>STRPPRFQRDFVDLRTDCPSTHPPIRVMQWNILAQALGEGKDNFVQCPVEALKWEERKCLILEEILAYQPDILCLQEVDHYFDTFQPLLSRLGYQGTFFPKPWSPCLDVEHNNGPDGCALFFLQNRFKLVNSANIRLTAMTLKTNQVAIAQTLECKESGRQFCIAVTHLKARTGWERFRSAQGCDLLQNLQNITQGAKIPLIVCGDFNAEPTEEVYKHFASSSLNLNSAYKLLSADGQSEPPYTTWKIRTSG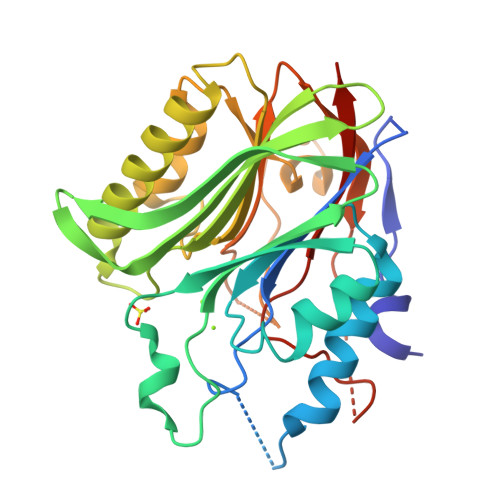ECRHTLDYIWYSKHALNVRSALDLLTEEQIGPNRLPSFNYPSDHLSLVCDFSFTEESDGLS[2x]Here we used a sequential symmetry expansion and relaxation approach to resolve the first asymmetric reconstruction of the ARV ICP by cryoEM to 3.3 Å. Lacking the outer capsid proteins VP5 and VP7, the ARV ICP retains the icosahedral, T = 2*, inner capsid shell composed of 60 asymmetric dimers of the 1214-residue, wedge-shaped, VP3 capsid shell proteins (CSPs) and 120 symmetrically arranged copies of the clamp protein (VP6) which form the ICP frame and provide support, respectively. Situated beneath 11 of 12 I5 vertices in ARV are TECs, heterodimers of RdRp and NTPase. Atop each I5 vertex sits a pentameric turret, composed of five copies of VP1 TPs with their axial channels reaching the nascent mRNA translocating pores of the TEC.

Within ICPs, several dsRNA segments interact with each TEC and these interactions stabilize segments, enabling improved visualization of their major and minor grooves as observed in other RNA viruses. Five major dsRNA segments are observed adjacent to each TEC and are labeled based on their positions relative to the TEC, with a 6th segment observed adjacent to the template entrance in polar vertices. VP3 dimers (containing conformers VP3A and VP3B) encircle each 5-fold vertex; with VP3A conformers seated around the 5-fold vertex center, creating pores adjacent to each transcriptional enzymatic complex’s (TEC’s) template exit channel for direct transcript capping and release via VP1 turret proteins (TPs). Absent conspicuous VP3 rearrangement, the internal volume of the ICP increased from 5.51 × 107 Å3 to 6.02 × 107 Å3, or about 9.3% relative to the grass carp reovirus (GCRV) virion and ISVP with which golden shiner reovirus (GSRV) shares 96%–100% a.a. sequence identity. By reducing the packaging density and thus viscosity of the genome, the enlarged ICP provides the rigid dsRNA segments greater freedom of movement and presumably reduces the energy required to initiate transcription. The VP2 RNA-dependent RNA polymerase (RdRp) is organized into the N-terminal domain (NTD), C-terminal bracelet (CTB), and RdRp core which is further differentiated into the thumb, fingers, and palm subdomains. Our RdRp structure reveals several local architectural changes within these RdRp channels when compared to the ISVP. Viewed down the template entry channel, a positively charged finger domain loop extends into the template entry channel in the ICP, widening to accommodate nucleic acids. From within the channel, the priming loop—thought to separate template and transcript strands—shifts away from the transcript exit channel and orients the catalytically important serine residues towards the would-be incoming template. This migration away from the CTB widens the mRNA exit channel, likely promoting exit through the adjacent I5 pores and turrets.

> EELFNALPQPLQQLSLALAGEIPLTDHIFEQAASTWHVQPRSLTYKLLDHIPFSTPVVVPPSIYHSLDWSKCFAVNQDRVERVPTIDDPDDVYVPNSDIGPLLTSLHTIPDYGFLHPAIENDATTLRAERARCASTFYKIASSQARQVKLDPIRMLGFLLLVQARPRVPSGLVTDQPTRRDPTQSPALHAIWQVMQYYKVAGVYYAPALVVPSGAIWWIPPPGKRNVVSVQYLLTDLINLAILAHMTDMSPTLELTGVLMYLRAASSHSHAYTLLQMKSVFPALSLRSMYRNKGFGGKAPAIEWTEPRSKYKFRWTGVTQLHDGLRPRSPSMDVPTLEVLTKYELVDIGHIIIRERNAHPRHNHDSVRFVRDVMALTSGMYLVRQPTMSVLREYSQVPDIKDPIPPSAWTGPIGNVRYLLPSVQGPARHLYDTWRAAARQIAQDPQWHDPLNQAIMRAQYVTARGGSSASLKFALKVTGIVLPEYDDSKVKKSSKIYQAAQIARIAFMLLIAAIHAEVTMGIRNQVQRRARSIMPLNVIQQAISAPHTLVANYINKHMNLSTTSGSVVTDKVIPLILYASTPPNTVVNVDIKACDASITYNYFLSVICGAMHEGFEVGNADAAFMGVPSTIVSDRRSSVAPYSRPISGLQTMVQHLADLYAAGFRYSVSDAFSSGNKFSFPTSTFPSGSTATSTEHTANNSTMMEYFLNVHAPSHVKSASLKRILTDMTIQRNYVCQGDDGILLLPHEAASKISADDMNELLTCLRDYGQLFGWNYDIDWSDTAEYLKLYALMGCRIPNTSRHPPVGKEYAAPQTDEIWPSLIDIVIGHHLNGVTDVLNWREWLRFSWAFACYSSRGGYTNPKGQSFSAQYPWWTFVYLGIPPILLPGQTPFIHSCYMPPGDQGMFSILNGWRDWLISHASTTLPPLRHNHPVWGLSDVPSLLSQFGVYAGYHAAQHYRRPKPAPETASSDSINQITSDLTEYLFYDSALKARVMKGRYNWERLSSSLSLNVGSRVPSLFDVPGKWVAAGRDAEKPPPSSVEDMFTSLNRCIRRPTHSFSRLLELYLRVHVTLGESIPLAIDPDVPQVAGADPANDDHWFKYTCLGDIPSATRNYFGESLFVGRVVSGLDVEAVDATLLRLKILGAPPEAFIAVLNGIGMSDSEAHQIAGRISLANAQLVQIARVVHLSIPSSWMTLNTGPYIHHHAYDFKPGITQPSAKSRDKSIWMSPILKLLCTSYAMTVAGPVRTSIVTEIDGSAAALSGNLRVWMRDV;> MITIVVIPTAHFSWTDTNFLNSVDYRLTSQPKIRDRFAVYAPGWLRRQLDEFSASLTASELLQALQTIPIPVKARCLLLPKPKRFAQWLLDVPSANIWHIPVTTLRATVASKHPSSDVYNYIPDHVPPSAEFDTVTRRVAAGRDIYVRSTKVLGAPLCLAAPAKYYAGYLSTHQLDGVYPDNWAPDNFHKREFCLTILPSLLGPRTFLLDVDADRDASYPLSVLWPQLRVLALKSRLLLPPVALLRRVVDPGLKPTWSADSDAAFRALRLSRPSSASKPTGFDFSALPVVDIICLFESEPDDHGRVAPGTRLTIHSVPTDLLTSLSIQEGVRYPLRQESGMFVPWVLLALLMSDDVTISGTRRSVKLETAHASARPFVHITVERCASARVVDVRGSPAMYANAVCLTLPKGSYKSTIIDTLPAMFSDLSILEQAAVIDSDALGDSLRPSFETQFLERLENLDPKLLDRAVASILSPASDTSDDAVTTVLDVFNALYREVMTPAQRSRLPLLTQQGRVLAFAHSDYELLSANIPIQVVRGSIPIDHVVNLLARRNRVGGTALQVLLDYCYRTQASPLAPTPAGRLYKQLFGPWLMVPRLSDPLIKLRLVASAPAKVLRAAGWTIDGDPPLEVSCLCAYVTDRAMAAALIERRLDSRALVNVGGDQLMFVEYAPPLPLVSIPRTFLLPVTYVVHWVSPQRVLLNGGNVSFTSGLEWTFDD;>DIITRPTSDSIAAVANATKPAAVVSDPQSMKVTPIVNPSSYVCNVCNARFSTMSALSEHLRSDHRDDASTLLATPMINNAIRSFLTAWDGIRILSPDVSSKHLSAYLDSAVANGPELIVEDTGLCTSFMLLDNIPSAHLTKELIGFTWFMQMYQMTPPLPEGAVNRIVCMTNWASLGDEGRGLEVRLPPPTDSSVHAYKTVLSRGYIDNAQFNPLALRSNVLLMLLQFTLSNLKINKSSTFTSDVTTITSGRMIRAFEGRPELLALAYPGRAVLPTQTKNAQFLSTAIADRIGRLDRANLIGGEVSAMVECMELCDALTLHIRETYVMLLRSMHQDPTQIVQIVNECANNLLNSTIPISLRPTILCPWFASSEDLRLQQVMHLVNISSNTAAALPLVEALSTLLRSVTPLVLDPTVLTNAITTISESTTQTISPISEILRLLQPMGNDYAAFWKCIASWAYNGLVTTVLSEDAFPDSSQSITHLPSMWKCLFLTLAGPMTSDPHSPVKVFMALANLLAQPEPIAIGVPGMHQTTPASQFSHPGVWPPGFLNPQLINPQQAPLLRAFAEHIRANWPQPSEFGYGSTLQGSANLFIPPNRMVYPWPNQPLPRLTVAPTYDSAMSNWISTTIAFFIRVVNSVNMTATVNDLTRRTMTGVMTAMRQVKTMTPFYIQHMCPTELSVLASVTVTPPFQVPFTRLVQNDVITNVLVARVDPAQRGDAAVDIRATHATFAAALPVDPAAIVVAMLCGQTETNLIPSHHYGKAFAPLFASNAMFTRNQRAVITREAFVCARSAVAQCQDAGFLVPRPLDALRQFDVTSAAAAEIMHAVNDAFKTAFDLDGALLDGLALYGDPRIADLSAAYLQYGGNVVREHVPPGPSHIHRTLQQVESTFMAEMNLFNVARGNLYLVQTATNGNWSPMAPVAAPPFVRGGPNVRVVGRFGTIVPRPDGLEPQLIDDGNVPRDIAGDWVYPSDVLQVSVAVFCDYVWPMVKAGRTRVLVELGHYVYTLHYYDPQISLDEAPILEEWLSKINPAGIPPVPFCIPIPQVYPCITARRVHYAFTSENNNDSLFSTNAASIDTAFGENAAVSPLRWPGLVDPNYRVGTNDLPNRITLYNSLYRYNFTYPTLDGIMYVRSAT[10x];>[5x]TASPADTNVVPAKDAPTTNSPPSTTSPNQAAADANQQQAGIVSSQSGPNAVGDSAPSTSVNNDGDIITRPTSDSIAAVANATKPAAVVSDPQSM;>AQRQFFGLTYNFYGQPAPLFDLNDLQELAGCYARPWTSRFSHLAISTGSLPVWSARYPSVASRNIIVNTLLGAHLNPFAGGQVTSHQGITWRDPVLSSLAPVPAIQPPPVWAVAENVPLDSNNYPTYVLNLSSMWPINQDVHIMTMWALSDQGPIYHLEVPVDPMPAATTAALMAYIGVPIAHLAQTAYRFAGQLPQSPDSTMVSTIRWLSAIWFGSLTGRLNRSRTCNGFYFEFAKPALNPDQAVLKWNDGARAAPPAAAQSSYMRCISPHWQHQIVEVAGALMSQSVTAVTGLPALIDEATLPAWSQGVANLTGNGQGVVPCLDYNPVPMAAARHLQWRQDGLITAAQEAQLNNDYTAYALTIERHLTAMLVANPIAAGRMPIQPFNAADFGQAGQTAAAVALAQAMFV[10x];>AAVFGIQLVPKLNTSTTRRTFLPLRFDLLLDRLQSTNLHGVLYRALDFNPVDRSATVIQTYPPLNAWSPHPAFIENPLDYRDWTEFIHDRALAFVGVLTQRYPLTQNAQRYTNPLVLGAAFGDFLNARSIDIFLDRLFYGPTQESPITSITKFPYQWTIDFNVTADSVRTPAGCKYITLYGYDPSRPSTPATYGKHRPTYATVFYYSTLPARSRLLANLAAGPTVLEHFDSPTYGPHLLLPQTGDVLGYSSSLISQAALLMVESVMDALRDNANASASTAVTRLDQSYHPVTSFDPSTFNTLLQRATNLALLAVQGVQSESAIPAIPTMSDVRSFVARLMAEGDPQQWFPYRVDQILYWPESPFVPPIGPFYAPFRPVNFPFTTGSYTVVPDASRPLRLLPQYRNATITVQQADDAYEDTALSPLITTHGFCVTGGVSTSIYDISGDPTAYPPAQLVDTPNDYFDRERMARRDLFRRLRAPADRSAIKDRAVFDFLASLVNPTTANPVLDTSFSMAYLGASSAHANADEPVILADIRSGSIPGLPIPRRIVQFGYDVVHGSLLDLSRAVPTGTFGLVYADLDQVEDAGTDMPAANRAAIAMLGTALQMTTAGGVSVLKVNFPTRAFWTQVFNLYATHATTLHLVKPTIVNSSEVFLVFGGRQSNGALRSTTALQRALLSLYARNAAIDRAVTHIPFFGVPDDGTSDLGIDAVRLFDPMFSDAVANLPSNALASLVSRVVPSSIMFTRVPSNGPVSTTIYGKRTFLSNRRRARLRDVPMLITTTLVHQRRFTTPPTFTLFSSEAVPVTTLVAAGYNSFISEQTRNPNLAHLLDLGTGPECRILSLIPPTLQVTMSDARPCAELMASFDPALTAYVQGDYSTAAFWNGIRCDSATAIFTLGAAAAAAGTDLIAFVQQLIPRIVAAGGTRMWLQLNTPLYEVSSLPDLIDIDLRDRVYRFNGGERVEPYADPVPLQQAIAALLPAAALSWHTLSPTCDWLPYIIGVGSPLNLSDINTAISYSRLTPILHIDTTTPPLRVNPVPTPLNQQCAIRITSLDPAAVLSVQHNGVEVIGGTPGNVISVAGAAALQYILANQEFLLQFTPTLPGIFDVFLTTLGQPPVPRGSFTITPPPTTVVLNMPPPGQLDFTDVGNDARITCDPYYQLAVCIFKDGQYVRVNPEKASVVTNAPNRDLHFVLDLADNHVLLYLCDVTPSGLGDRIAFPIVDIYRIAFPRNTPVRASLPYTGGGAHLTSGGNPFMSLTTPPAVLPAGVALAALSTSVATQYPTYTLPAGVYEYVI[5x]> AFVVTDNCIKCKYTDCVE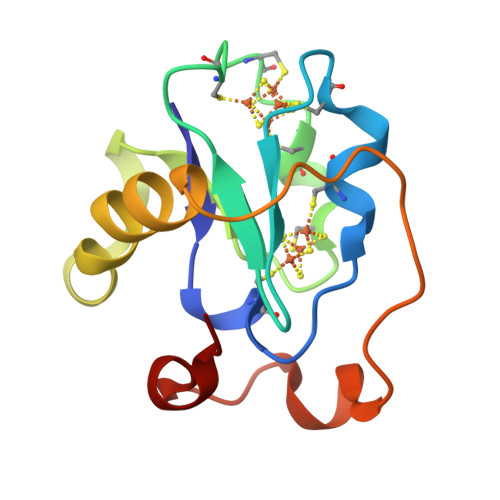VCPVDCFYEGPNFLVIHPDSCIDCALCEPECPAQAIFSEDEVPEDMQEFIQLNAELAEVWPNITEKKDPLPDAEDWDGVKGKLQHLER CHD4 is an essential, widely conserved ATP-dependent translocase that is also a broad tumour dependency. In common with other SF2-family chromatin remodelling enzymes, it alters chromatin accessibility by repositioning histone octamers. Besides the helicase and adjacent tandem chromodomains and PHD domains, CHD4 features 1000 residues of N- and C-terminal sequence with unknown structure and function. Auto-inhibition is relieved by a previously unrecognized C-terminal SANT-SLIDE domain split by ~150 residues of disordered sequence, most likely by binding of this domain to substrate DNA.

After generating many constructs covering the region 1200–1912, we were able to successfully express and purify a protein comprising residues 1380–1810, but lacking residues 1552–1689. These residues form part of what is predicted by PONDR25 to be a disordered segment of ~160 residues in length (residues 1540–1700). We determined the three-dimensional structure of this polypeptide by X-ray crystallography to a resolution of 2.9 Å. Furthermore, our X-ray crystal structure of C1bC2a reveals a SANT-SLIDE domain that closely resembles the structure observed in both CHD1 and ISWI. First, no clear electron density was observed for the residues that constitute the bulk of the second helix of the SANT domain (α2 in human CHD1). Second, a β-hairpin that links α3 and α4 in human CHD1 has ‘relocated’ to a position N-terminal to the first helix in hCHD4; Fig. 5B shows the high sequence similarity between these two elements. Third, the SLIDE domain features an additional N-terminal helix in hCHD4. The most obvious difference, however, is the absence of electron density for the extended linker sequence (which is 60 residues in length in the truncated construct used for crystallization). To test this hypothesis, we titrated 46w60 nucleosomal DNA (without histones) with purified CHD4(1380–1810) in an MST experiment. Figure 5C shows that WT C1bC2a can bind DNA with micromolar affinity, consistent with our hypothesis that the C-terminal region of CHD4 harbours a SANT-SLIDE like DNA-binding domain.

>RSEAPRRPSRKGLRNDKDKPLPPLLARVGGNIEVLGFNARQRKAFLNAIMRYGMPPQDAFTTQWLVRDLRGKSEKEFKAYVSLFMRHLCEPGADGAETFADGVPREGLSRQHVLTRIGVMSLIRKKVQEFEHVNGRWSMPELAEVEENKKMSQPGSPSPKTPTPSTPGDTQPNTPAPVPPAEDGIKIEENSLKEEESIEGEKEVKSTAPETAIECTQAPAPASEDEKVVVEPPEGEEKVEKAEVKERTEEPMETEPKGAADVEKVEEKSAIDLTPIVVEDKEEKKEEEEKKEVMLQNGETPKDLNDEKQKKNIKQRFMFNIADGGFTELHSLWQNEERAATVTKKTYEIWHRRHDYWLLAGIINHGYARWQDIQNDPRYAILNEPFKGEMNRGNFLEIKNKFLARRFKLLEQALVIEEQLRRAAYLNMSED[2x]>[4x]KITGLLDGDRVIVFDKNGISKLS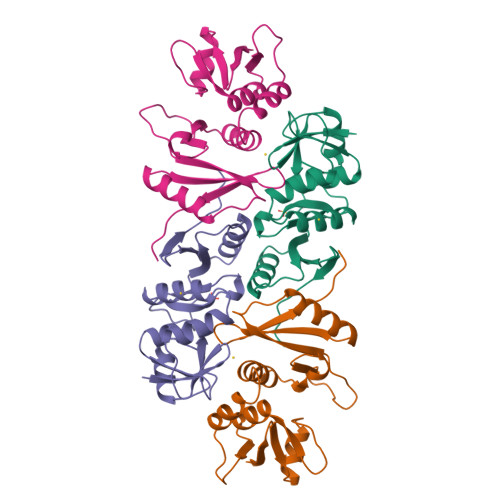ARHYGNVEGNFLSLSLVEALYLINLGWLEVKYKDNKPLSFEELYEYARNVEERLCLKYLVYKDLRTRGYIVKTGLKYGADFRLYERGANIDKEHSVYLVKVFPEDSSFLLSELTGFVRVAHSVRKKLLIAIVDADGDIVYYNMTYVKP>MGSTTTLENPALLGWFRGQQTPEGWFDLLALIVDGMVRNVGELESQPFLRQMGIALADQYPLPASETVGELEANINAQLARFGWGCVEIDTSDTDLTLRHQALPVSRVEDQQSRWCHAFCAILEGLYVRWMQGQGGKSHVTVSRERLFS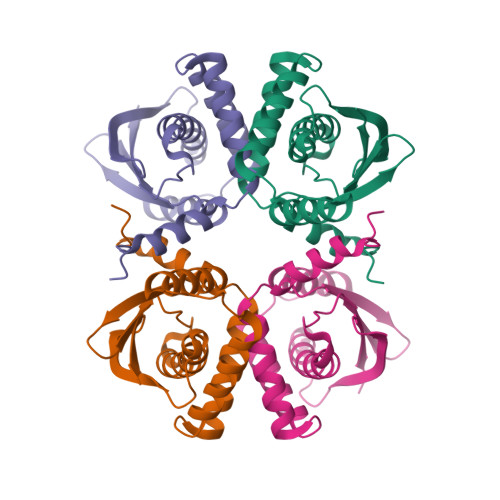LSDVQFRYHNPQ[4x]>EQDIYLPIAN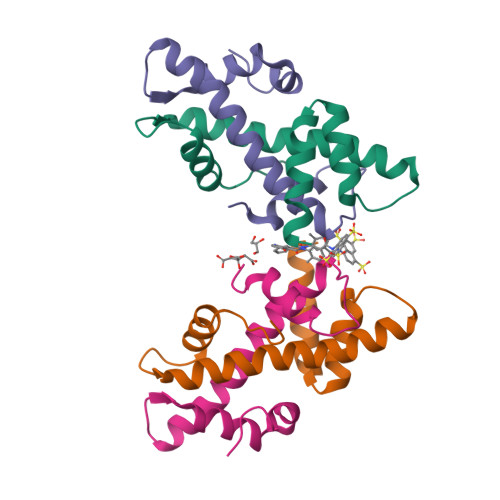VARIMKNAIPQTGKIAKDAKECVQECVSEFISFITSEASERCHQEKRKTINGEDILFAMSTLGFDSYVEPLKLYLQKFR[2x];>QELPLARIKKIMKLDEDVKMISAEAPVLFAKAAQIFITELTLRAWIHTEDNKRRTLQRNDIAMAITKFDQFDFLIDIVPR[2x]>MTSRKKVLLKVIILGDSGVGKTSLMNQYVNKKFSNQYKATIGADFLTKEVMVDDRLVTMQIWDTAGQERFQSLGVAFYRGADCCVLVFDVTAPNTFKTLDSWRDEFLIQASPRDPENFPFVVLGNKIDLENRQVATKRAQAWCYSKNNIPYFETSAKEAINVEQAFQTIARNALKQETEVELYNEFPE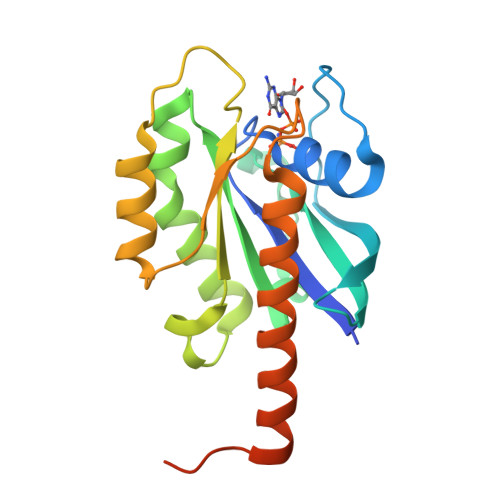PIKLDKNERAKASAESCSC[4x]> YVDRRRGVSSETTVEIHSPSKVVKKQLNPETKARIEKCLRGNILFRSLGEDSLEVVYSSMFEKTAEAGHFIMKQYDEGDNFYVIESGTCNILIQPNPDAEPVHKSTIGPGASFGELALMYGTPRAASVQAVSNVRLWALDRDTFRRILLTQTMRKRRQYEDFLAQVPLFEALTSYERMTM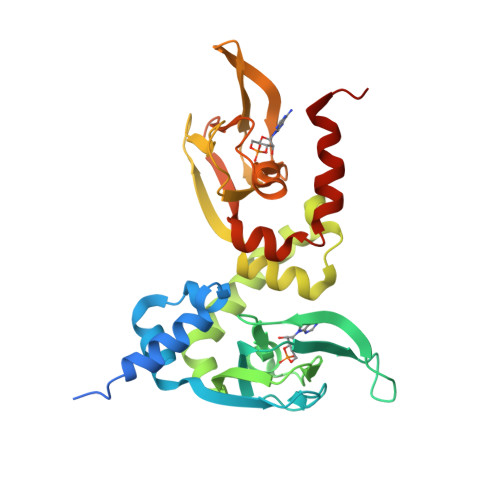ADALQPCTFKDKEIVVKEGEDGGSFYIIIDGKMKVNQTLNGRIHTINILGPKDFFGEMSLMFNQPCVATVVSEGVSHCVSLDRESFTALLGPMEEILQRNMQNYSAPREEVQE2-(benzoylamino)-2-deoxy-beta-D-glucopyranose 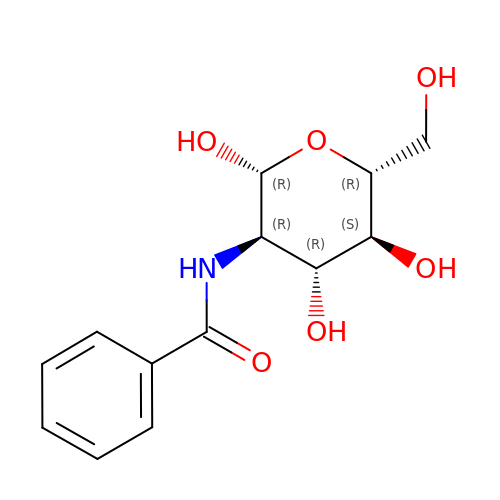| C13 H17 N O6 | VSGKVJPCJOJUBP-VDWIVTDKSA-N> SYSTLANFPVQARNDNISPWTITGFADAESSFMLTVSKDSKRNTGWSV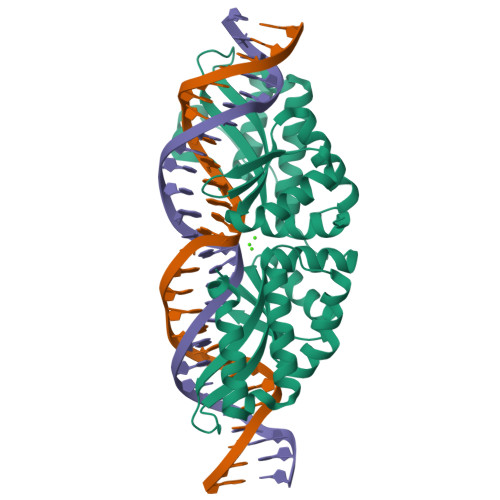RPRFRIGLHNKDVTILKSIREYLGAGIITSDIDARIRFESLKELEVVINHFDKYPLITQKRADYLLFKKAFYLIKNKEHLTEEGLNQILTLKASLNLGLSEELKEAFPNTIPAERLLVTGQEIPDSNWVAGFTAGEGSFYIRIAKNSTLKTGYQVQSVFQITQDTRDIELMKNLISYLNCGNIRIRKYKGSEGIHDTCVDLVVTNLNDIKEKIIPFFNKNHIIGVKLQDYRDWCKVVTLIDNKEHLTSEGLEKIQKIKEGMNRGRSL> AQSVPYGVSQIKAPALHSQGYTGSNVKVAVIDSGIDSSHPDLKVAGGASMVPSETNPFQDNNSHGTHVAGTVAALNNSIGVLGVAPSASLYAVKVLGA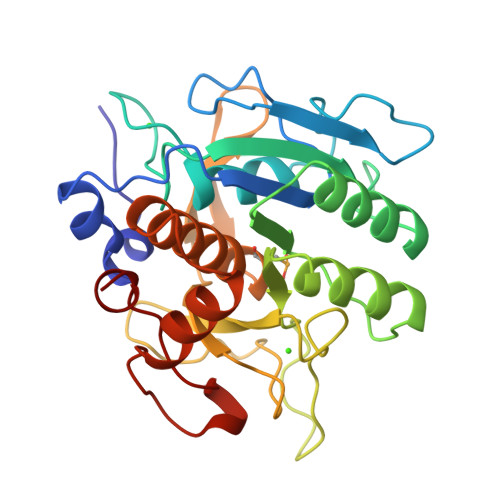DGSGQYSWIINGIEWAIANNMDVINMSLGGPSGSAALKAAVDKAVASGVVVVAAAGNEGTSGSSSTVGYPGKYPSVIAVGAVDSSNQRASFSSVGPELDVMAPGVSIQSTLPGNKYGAYNGTUMASPHVAGAAALILSKHPNWTNTQVRSSLENTTTKLGDSFYYGKGLINVQAAAQ RNA helicase DDX21 plays vital roles in ribosomal RNA biogenesis, transcription, and the regulation of host innate immunity during virus infection. DDX21 is composed of three domains, including the N‐terminal domain, the middle D1 and D2 domain, and the C‐terminal foldase domain. In summary, here we reported multiple sets of crystal structures of RNA helicase DDX21 either in ligand‐free (DDX21‐apo) or in complex with AMP (DDX21‐AMP), ADP (DDX21‐ADP), or a nonhydrolyzable ATP analog (AMPPNP) and a 15‐nucleotide poly(U) ssRNA (DDX21‐AMPPNP‐U15), corresponding to different unwinding states (except for DDX21‐AMP). We elucidated the conformational rearrangements upon the ATP and ssRNA binding during the dsRNA unwinding cycle, and described an RNA unwinding machinery including one wedge helix, one sensor motif V, and the DEVD box.

To better understand the RNA recognition and unwinding mechanism of DDX21, we determined the crystal structure of human DDX21 helicase core (residue 188–563), encompassing the conserved RecA‐like helicase core domains D1 and D2 in complex with AMPPNP and a 15‐mer poly(U) ssRNA at 2.24 Å resolution, which represents a post‐unwound or pre‐hydrolysis state in the unwinding cycle. The DDX21‐AMPPNP‐ssRNA ternary complex structure contained two molecules in the asymmetric unit, named as A chain and B chain, respectively, which bound to a poly(U) mRNA mimic, a non‐hydrolyzable nucleotide AMPPNP, and one Mg2+ ion. The complex structure revealed a canonical DEAD box RNA helicase core closure process, which brought the N‐terminal ATPase and C‐terminal helicase in close vicinity to create the functional ATPase site and the nucleotide‐binding cleft. The two domains (D1 and D2) of DDX21 clasped ssRNA, enfolding it within an interaction network that was dominated by polar contacts. DDX21 formed eleven hydrogen bonds with the phosphate groups of the RNA backbone and recognized six 2’‐OH groups of RNA backbone, which thereby discriminated against DNA substrates. Uniquely, Gln352 recognized both the base moieties and 2’‐OH group of U4, which was not found in other DEAD‐box proteins. Thus the RNA was bent between U4 and U5, and the bent region was located near the DDX21 motif Ic within the conserved α6 helix, the so‐called “wedge” helix. The presumptive attacking water for ATP hydrolysis was close to the γ‐phosphorus atom of AMPPNP and interacted with the side chains of Glu340 (motif II) in the D1 domain, His523 (motif VI) and the amide group of Gly500 (motif Va) in D2 domain. More importantly, only in the AMPPNP‐bound form, the residues Asp339 and Glu340 within the DEVD box bound to the γ‐phosphorus atom through Mg2+ ion and water molecules, and incorporated with multiple inter‐domain interactions. The interactions, in turn, established more contacts with the presumptive attacking water and stabilized the interactions with γ‐phosphorus.

>[2x]SFSNFPISEETIKLLKGRGVTFLFPIQAKTFHHVYSGKDLIAQARTGTGKTFSFAIPLIEKLHGELQDRKRGRAPQVLVLAPTRELANQVSKDFSDITKKLSVACFYGGTPYGGQFERMRNGIDILVGTPGRIKDHIQNGKLDLTKLKHVVLDEVDQMLDMGFADQVEEILSVAYKKDSEDNPQTLLFSATCPHWVFNVAKKYMKSTYEQVDLIGKKTQKTAITVEHLAIKCHWTQRAAVIGDVIRVYSGHQGRTIIFCETKKEAQELSQNSAIKQDAQSLHGDIPQKQREITLKGFRNGSFGVLVATNVAARGLDIPEVDLVIQSSPPKDVESYIHRSGRTGRAGRTGVCICFYQHKEEYQLVQVEQKAGIKFKRI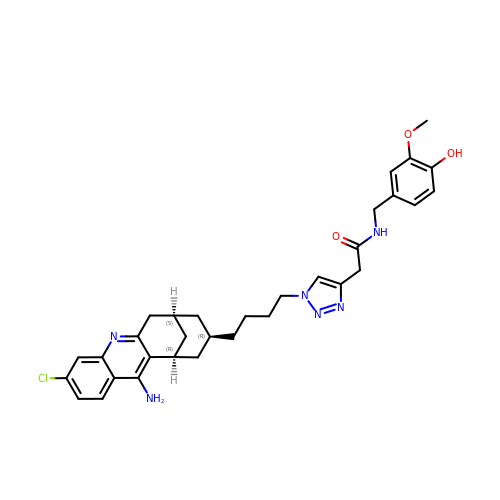2-{1-[4-(12-Amino-3-chloro-6,7,10,11-tetrahydro-7,11-methanocycloocta[b]quinolin-9-yl)butyl]-1H-1,2,3-triazol-4-yl}-N-[4-hydroxy-3-methoxybenzyl]acetamide | C32 H37 Cl N6 O3 | ACGLNWGWENJFEC-BAGYTPMASA-N>ANPLYQKHIISINDLSRDDLNLVLATAAKLKANPQPELLKHKVIASCFFEASTRTRLSFQTSMHRLGASVVGFSDSANTSLGKKGETLADTISVISTYVDAIVMRHPQEGAARLATEFSGNVPVLNAGDGSNQHPTQTLLDLFTIQQTEGRLDNLHVAMVGDLKYGRTVHSLTQALAKFDGNRFYFIAPDALAMPEYILDMLDEKGIAWSLHSSIEEVMAEVDILYMTRVQKERLDPSEYANVKAQFVLRASDLHNAKANMKVLHPLPRVDEIATDVDKTPHAWYFQQAGNGI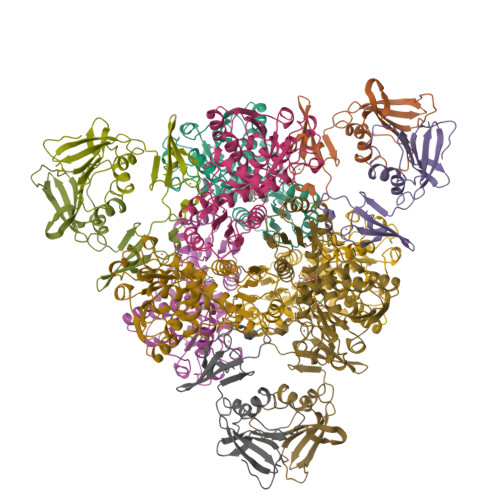FARQALLALVLNRDLVL[2x];>MTHDNKLQVEAIKRGTVIDHIPAQIGFKLLSLFKLTETDQRITIGLNLPSGEMGRKDLIKIENTFLSEDQVDQLALYAPQAAVNRIDNYEVVGKSRPSLPERIDNVLVCPNSNCISHAEPVSSSFAVRKRANDIALKCKYCEKEFSHNVVLAN[2x]> FACKTANGTAIPIGGGSANVYVNLAPAVNVGQNLVVDLSTQIFCHND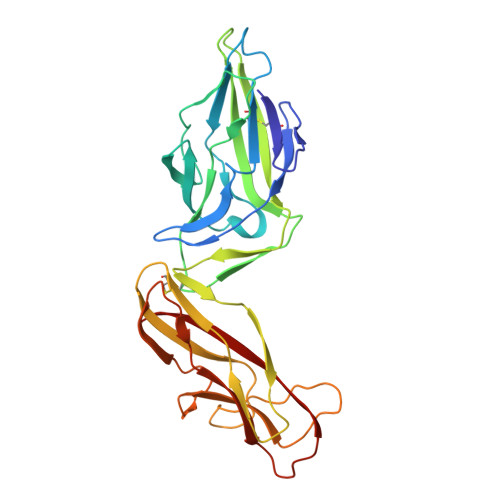YPETITDYVTLQRGSAYGGVLSSFSGTVKYNGSSYPFPTTSETPRVVYNSRTDKPWPVALYLTPVSSAGGVAIKAGSLIAVLILRQTNNYNSDDFQFVWNIYANNDVVVPTGGCDVSARDVTVTLPDYPGSVPIPLTVYCAKSQNLGYYLSGTTADAGNSIFTNTASFSPAQGVGVQLTRNGTIIPANNTVSLGAVGTSAVSLGLTANYARTGGQVTAGNVQSIIGVTFVYQ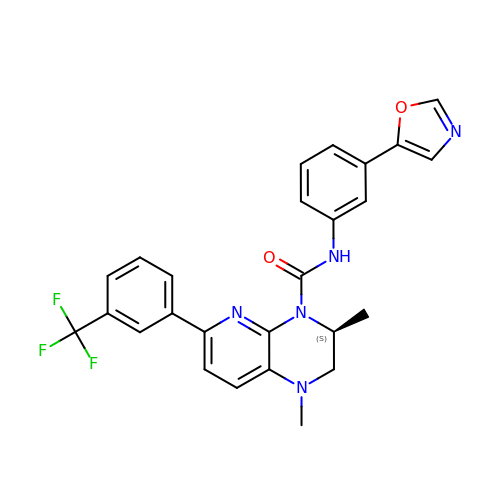(3S)-1,3-dimethyl-N-[3-(1,3-oxazol-5-yl)phenyl]-6-[3-(trifluoromethyl)phenyl]-2,3-dihydropyrido[2,3-b]pyrazine-4(1H)-carboxamide | C26 H22 F3 N5 O2 | NWNBKQCPAUNKSG-INIZCTEOSA-N> LCTPSRA;> LAHSKMVPIPAGVFTMGTDDPQIKQDGEAPARRVTIDAFYMDAYEVSNTEFEKFVNSTGYLTEAEKFGDSFVFEGMLSEQVKTNIQQAVAAAPWWLPVKGANWRHPEGPDSTILHRPDHPVLHVSWNDAVAYCTWAGKRLPTEAEWEYSCRGGLHNRLFPWGNKLQPKGQHYA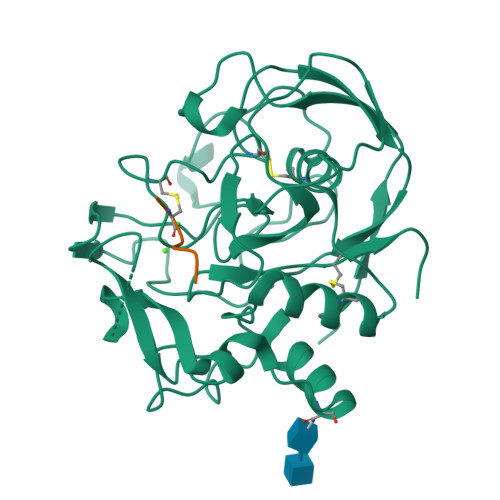NIWQGEFPVTNTGEDGFQGTAPVDAFPPNGYGLYNIVGNAWEWTSDWWTVHHSVEETLNPKGPPSGKDRVKKGGSYMSHRSYCYRYRCAARSQNTPDSSASNLGFRCAADRLP> SWRHIRAEGLDSSYTVLFGKAEADEIFQELEKEVEYFTGALARVQVFGKWHSVPRKQATYGDAGLTYTFSGLTLSPKPWIPVLERIRDHVSGVTGQTFNFVLINRYKDGSDHIGEHRDDCRELAPGSPIASVSFGASRDFVFRHKDSRGKSPSRRVAVVRLPLAHGSLLMMNHPTNTHW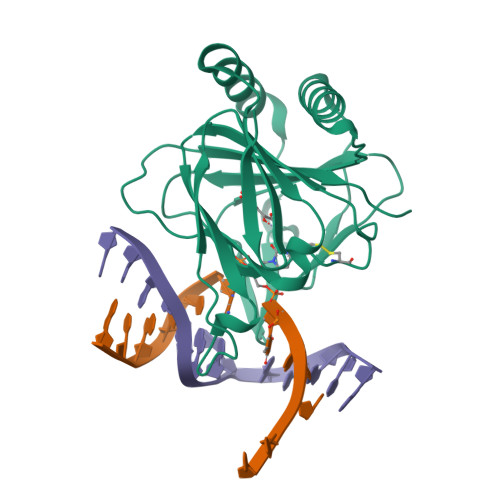YHSLPVRKKVLAPRVNLTFRKILL>[7x]SLGSDADSAGSLIQPMQIPGIIMPGLRRLTIRDLLAQGRTSSNALEYVREEVFTNNADVVAEKALKPESDITFSKQTANVKTIAHWVQASRQVMDDAPMLQSYINNRLMYGLALKEEGQLL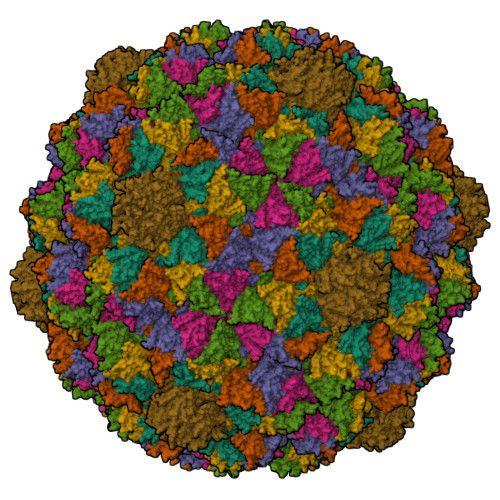NGDGTGDNLEGLNKVATAYDTSLNATGDTRADIIAHAIYQVTESEFSASGIVLNPRDWHNIALLKDNEGRYIFGGPQAFTSNIMWGLPVVPTKAQAAGTFTVGGFDMASQVFDRMDATVEVSREDRDNFVKNMLTILCEERLALAHYRPTAIIKGTFSSGS>SDLQRLKFIRHARQLGFSLESIRELLSIRIDPEHHTCQESKGIVQERLQEVEARIAELQSMQRSLQRLNDACCGTAHSSVYCSILEALEQ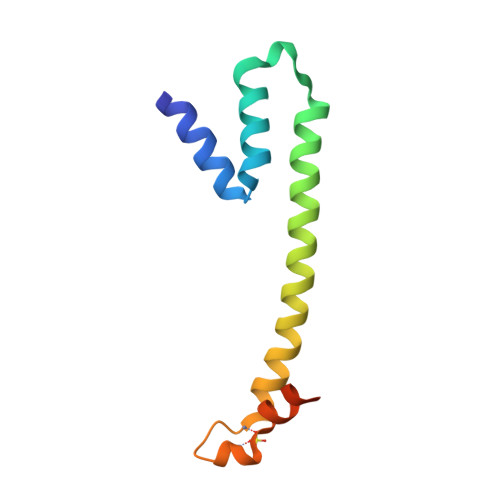GASGVKSGC[2x]> GPGSMSASQDSRSRDNGPDGMEPEGVIESNWNEIVDSFDDMNLSESLLRG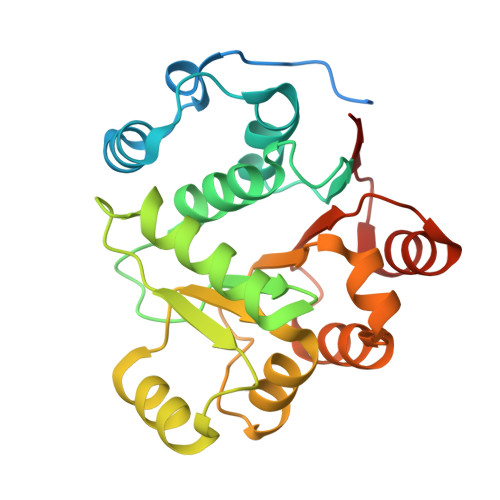IYAYGFEKPSAIQQRAILPCIKGYDVIAQAQSGTGKTATFAISILQQIELDLKATQALVLAPTRELAQQIQKVVMALGDYMGASCHACIGGTNVRAEVQKLQMEAPHIIVGTPGRVFDMLNRRYLSPKYIKMFVLDEADEMLSRGFKDQIYDIFQKLNSNTQVVLLSATMPSDVLEVTKKFMRDPIRILVKK> CDNSSSSSTSGSPGSPGNPGNPGTPGTPDPQDVVVRLPDVAVPGEAVQASARQAVIHLVDIAGITSSTPADYATKNLYLWNNETCDALSAPVADWNDVSTTPTGSDKYGPYWVIPLTKESGCINVIVRDGTNKLIDSDLRVSFSDFTDRTVSVIAGNSAVYDSRADAFRAAFGVALADAHWVDKTTLLWPGGENKPIVRLYYSHSSKVAADSNGEFSDKYVKLTPTTVNQQVSMRFPHLASYPAFKLPDDVNVDELLQGETVAIAAESDGILSSATQVQTAGVLDDTYAAAAEALSYGA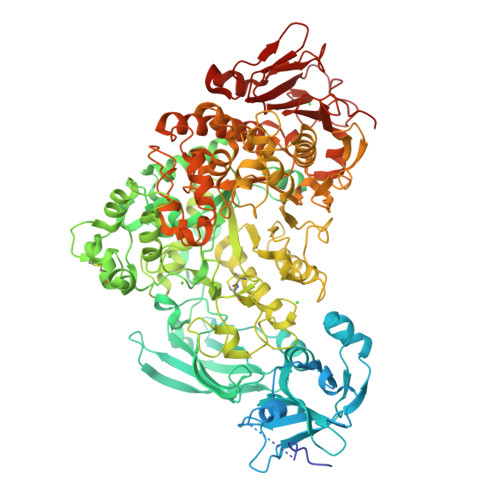QLTDSGVTFRVWAPTAQQVELVIYSADKKVIASHPMTRDSASGAWSWQGGSDLKGAFYRYAMTVYHPQSRKVEQYEVTDPYAHSLSTNSEYSQVVDLNDSALKPEGWDGLTMPHAQKTKADLAKMTIHESHIRDLSAWDQTVPAELRGKYLALTAQESNMVQHLKQLSASGVTHIELLPVFDLATVNEFSDKVADIQQPFSRLCEVNSAVKSSEFAGYCDSGSTVEEVLTQLKQNDSKDNPQVQALNTLVAQTDSYNWGYDPFHYTVPEGSYATDPEGTARIKEFRTMIQAIKQDLGMNVIMDVVYNHTNAAGPTDRTSVLDKIVPWYYQRLNETTGSVESATCCSDSAPEHRMFAKLIADSLAVWTTDYKIDGFRFDLMLYHPKAQILSAWERIKALNPDIYFFGEGWDSNQSDRFEIASQINLKGTGIGTFSDRLRDAVRGGGPFDSGDALRQNQGVGSGAGVLPNELTTLSDDQARHLADLTRLGMAGNLADFVLIDKDGAVKRGSEIDYNGAPGGYAADPTEVVNYVSKHDNQTLWDMISYKAAQEADLDTRVRMQAVSLATVMLGQGIAFDQQGSELLRSKSFTRDSYDSGDWFNRVDYSLQDNNYNVGMPRSSDDGSNYDIIARVKDAVATPGETELKQMTAFYQELTALRKSSPLFTLGDGATVMKRVDFRNTGADQQTGLLVMTIDDGMQAGASLDSRVDGIVVAINAAPESRTLQDFAGTSLQLSAIQQAAGDRSLASGVQVAADGSVTLPAWSVAVLELPQGESQGAGLPVSSK>[6x]LKESYLEESCSTITEGYLSVLRTGWYTNVFTLEVGDVENLTCADGPSLIKTELDLTKSALRELRTVSADQLAREEQIENPRQSKKRKRR;>VATAAAVTAGVA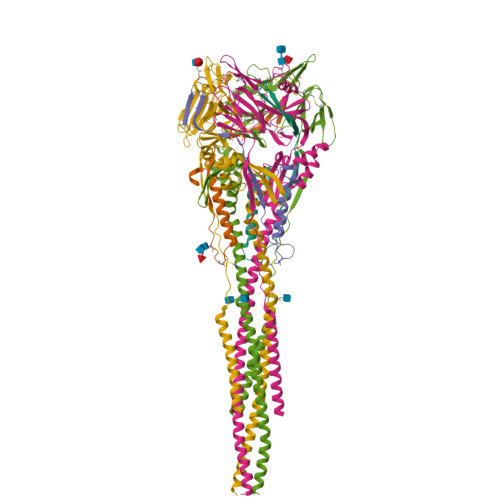IAKTIRLESEVTAIKNALKKTNEAVSTLGNGVRVLATAVRELKDFVSKNLTRAINKNKCDIADLKMAVSFSQFNRRFLNVVRQFSDNAGITPAISLDLMTDAELARAVSNMPTSAGQIKLMLENRAMVRRKGFGILIGVYGSSVIYMVQLPIFGVIDTPCWIVKAAPSCSEKKGNYACLLREDQGWYCQNAGSTVYYPNEKDCETRGDHVFCDTAAGINVAEQSKECNINISTTNYPCKVSTGRHPISMVALSPLGALVACYKGVSCSIGSNRVGIIKQLNKGCSYITNQDADTVTIDNTVYQLSKVEGEQHVIKGRPVSSSFDPVKFPEDQFNVALDQVFESIENSQALVDQSNRILSSAEKGNTSGRENLYFQ[6x]N-{4-[4-(2-amino-4-oxo-3,4-dihydro-5H-pyrrolo[3,2-d]pyrimidin-5-yl)butyl]-3-fluorothiophene-2-carbonyl}-L-glutamic 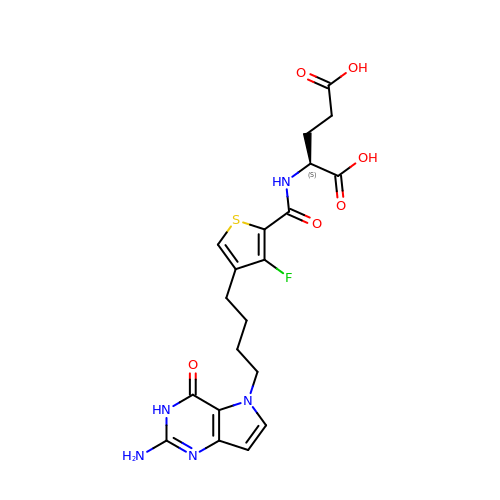acid | C20 H22 F N5 O6 S | HPZHEVFOCGGDJM-LBPRGKRZSA-N>[2x]MTDLKASSLRALKLMDLTTLKDDDTDEKVIALCHQAKTPVGNTAAICIYPRFIPIARKTLK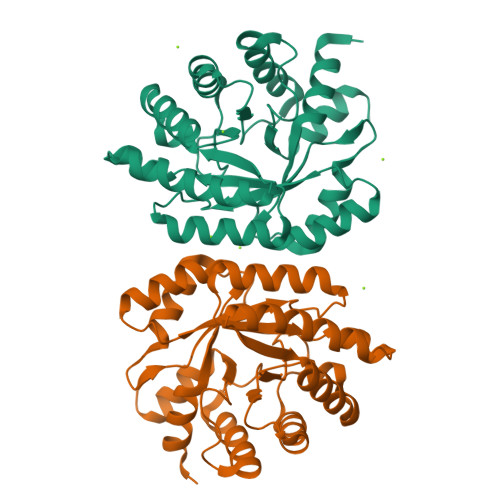EQGTPEIRIATVTNFPHGNDDIDIALAETRAAIAYGADEVDVVFPYRALMAGNEQVGFDLVKACKEACAAANVLLKVIIETGELKDEALIRKASEISIKAGADFIKTSTGKVAVNATPESARIMMEVIRDMGVEKTVGFKPAGGVRTAEDAQKYLAIADELFGADWADARHYRFGASSLLASLLKALGH> MSGFSTEERAAPFSLEYRVFLKNEKGQYISPFHDIPIYADKDVFHMVVEVPRWSNAKMEIATKDPLNPIKQDVKKGKLRYVANLFPYKGYIWNYGAIPQTWEDPGHNDKHTGCCGANAAIAVCEIGSKVCARGEIIGVKVLGILAMIDEGETDWKVIAINVDDPDAANYNDINDVKRLKPGYLEATVDWFRRYKVPDGKPENEFAFNAEFKDKDFAIDIIKS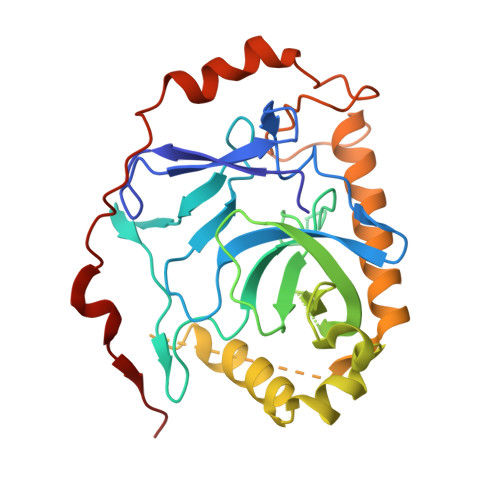THDHWKALVTKKTNGKGISCMNTTLSESPFKCDPDAARAIVDALPPPCESACTVPTDVDKWFHHQKN> PMTLGYWNIRGLAHSIRLLLEYTDSSYEEKKYTMGDAPDYDRSQWLNEKFKLGLDFPNLPYLIDGTHKITQSNAILRYIARKHNLCGESEKEQIREDILENQFMDSRMQLAKLCYDPDFEKLKPEYLQALPEMLKLYSQFLGKQPWFLGDKITFVDFIAYDVLERNQVFEPSCLDAFPNLKDFISRFEGLEKISAYMKSSRFLPRPVFTKMAVF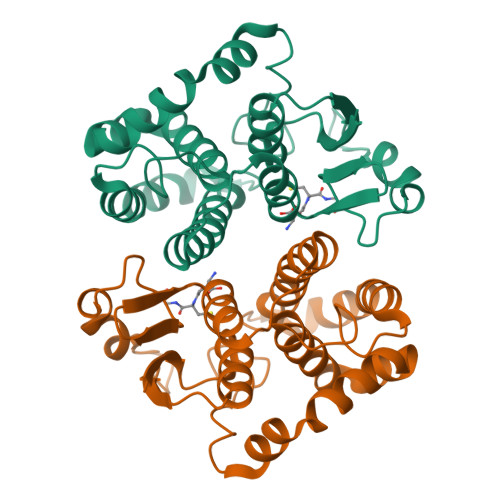GNK> MRILFLILLSFLNAFAFELVLNTGRENNQAFAVLHASNDLEFTCQKFITEAKVHFECDIVGMVDNKLKDQSFSAFDLKFIQEAQKIKMIILPKIQARMFDTSQNIYIDKELSSSSSHKSKAFTFIFTPELAPIKDYDGLDFNINFPHESLPYVGALDLNSDPVVIPQSADINTYLRIKKEYDKANYNQVVIDAQNAINRYRGSIFTSEFILYKLRAQNKLYTQDPSMRDQQILEKMIDDAKNWTRTFTSDKNFSEVLHIMLRTYIALAQRADVEYTMSILDNEQPNNYFTQLSKLDYADYIYNLNEKEKAVNIYENT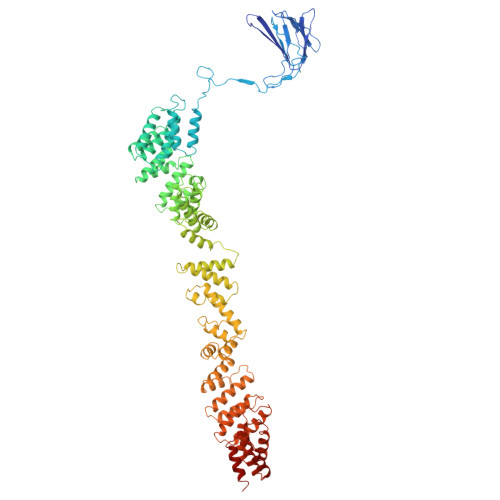YFNTKNLDLAARAAMSLAKNLLSNEQVNKAIEYINTILKANPEYFGKDIPRSLELAKLFNQKGQFDISASIYEDAFAKMSKLDPSYEETLKDLALVLSHANRSSDAKKYLDLYMDDYLDGKYLDEIKKASDEVFFALGDNNASFLHQRYTDLMKQYANKDENIANKALDEDVALYYKEGNFSAILAYKDLIESKKIPNATQFLEKAAINDLKNAIKADNCINAANIFMRFSAYDIGQKIENKKQMLACLIRTSNVEQALDYIDKNYNEDSIFYGLQKASILFDNKQYPQVIKISKDIANSRILKSDDENFKAYYLQFLSLLRLNDYNQAIKILQILESFPMNFSMVEAYDALLSYANDHNMQTTILTYAPKAIDYQNFKGINLFSPNLEFIYLDALTKINKNEESLAVLTDLLKLKLSDEDRARALYIQALTYERMQNIQAEKESLKQCLEIKSASNWQNLCKSKNQILNQ> GGASRSVIRSIIKSSRLEEDRKRYLMTLLDDIKGA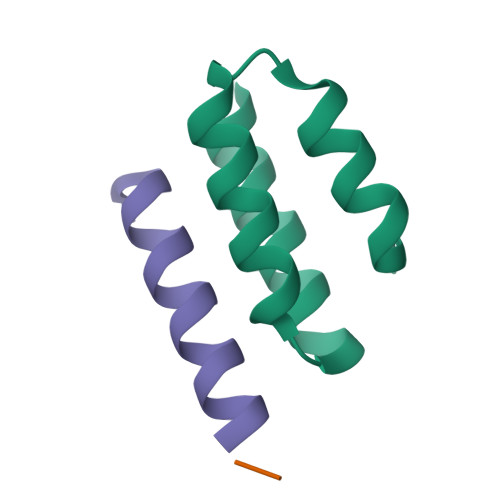NDLAKFHQMLMKIIMK;> QDSRRSADALLRLQAMAGIS;> GSGSGSGS> MQNLSKMQSRLHPRPEGEGGGGGGRTKEKGKSLQETHKEMLKNIESTNIGKPTIVEAQRILKIIDNLSTNLTIFIYLDSELISKFLDVAKHSKLSKDLVSKLSQRCLDLLKSQAEIEAKFKPYASLLDQSNKEAEDVEEEKMIDAERLRMQLENNFKDLVRHLRNSPEDFEIIKSMKTNVNPDLNDLVHCIHCQKVIMLKKLSTASEEDENHKAQLRDLEEKIEELEKKKNKIQEDLTKLKEHRQKFSKEKKEELEKLKNEIAEVKAEKEKKASQLKNELDNRLKQLERDHLAKKDKLDKELQKLEDDFAKLKQDHANDETKLKTNKRQQQNSLADNIESYDALMKDQHQKKQEIEEELAKIIEEVDTLKQLFKEIDEEKQRERELEEEFRLKKEQWEIQERRKKEAARCILHF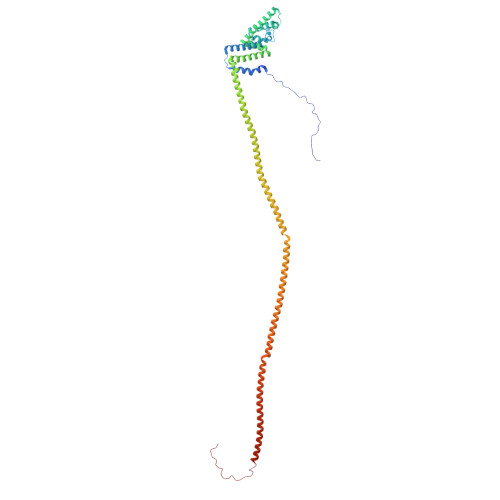LMARKEKSKKKKKKKGKKKK> MSVILASAGYDHTIRFWEALTGVCSRTIQHADSQVNRLEITSDKKYLAAAGHLHVRLYDIRSNN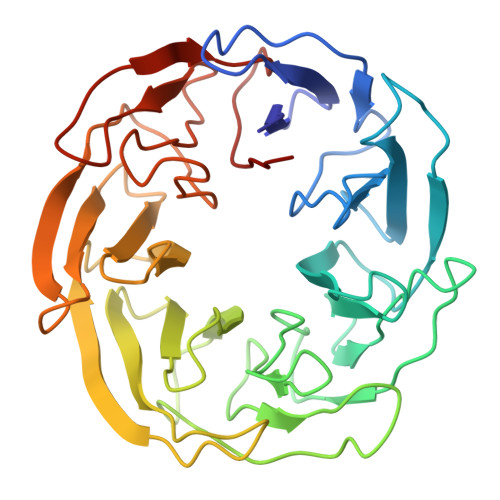PNPVSSFEGHKGNVTSIAFQQENRWMVSSSEDGTIKVWDVRSPSVQRNYKHNAPVNEVAIHPNQGELISCDQDGNIRIWDLGENQCTNQLTPEDNTPLQSLSVASDGSMLVAGNNKGNCYVWRMPHHTDASTLEPVTKFKSHTKYITRVLLSADVKNLATCSADHTARVWNIEDNYQLETTLDGHQRWVWDCAFSADSAYLVTACSDHYVRLWDLSTSEIVRQYGGHHKGAVCVALNDV> GSREREAGERRAQNACTLAAVTEKLGRAAELDYCDLEALHAELEPLARSADAAPQVEQFNELLTERARVPRRDLEHELLERRCDTELFVSTDDSVHELREKAGLLFQLSQLLLPEPRADQLWNFVCMANNFRIKFIYHFTSPSAESEQQSIENYFKFLDKYLSENLYKYMDIFEDESKGITRTLIHKQFINHILEPVREKVNVTMTKIAASNSASDVKMLVLLISEIFITDNALKKSHYYDGVGLVSLIDEAALEVWQNFEVESAVSQFEKLTTPGASLMS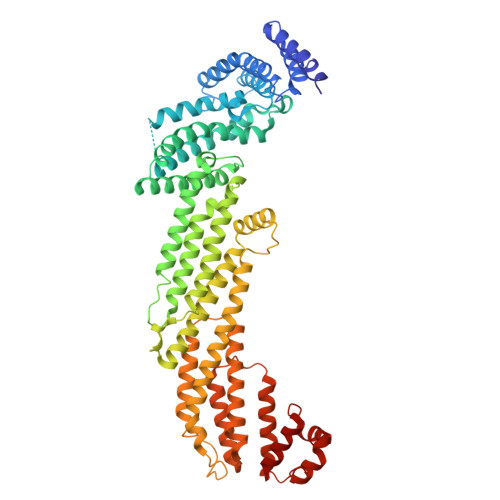PKNGADFGKLLENMYRYLEPFFSIDYRNLFSVKYQLVDEIFIQLPLKYRSFLLSKNILQNELTAEQQFENTCVKLHSLLLISNILVRFSHDFTFIEMTQQINKITDSDYEYIFDEVWESYDEAVIVLRDSIVHRWVKGLSSSLRNYFKYNEWDSIATAPEQCSAELVGALAWMKKMTDIFDKYWYPQHIIAQIKVALLENIIKFMLNYVVKLNKFSENGLRQLTFDYEALRATLGLPLEHSSVAEELALFEYFNILSMKYTNNKITSKFLDAEYVSSHHTRNFRELRESLQVSHLTSDEIADALYRTL>[2x]MSDLQQLFENNVRWAEAIKQEDPDFFAKLARQQTPEYLWIGCSDARVPANEIVGMLPGDLFV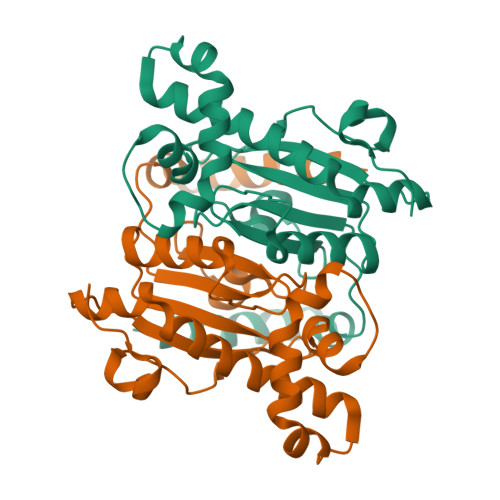HRNVANVVLHTDLNCLSVIQFAVDVLKVKHILVTGHYGCGGVRASLHNDQLGLIDGWLRSIRDLAYEYREHLEQLPTEEERVDRLCELNVIQQVANVSHTSIVQNAWHRGQSLSVHGCIYGIKDGLWKNLNVTVSGLDQLPPQYRLSPLGGCC> VKVDLESKRYGEKLKEVFLMLDNNVVECIKEITESSRNGKLVFFVGAGVSTLSDYPQWWRLVDKYHEELYGSPKKGNYSSDEYLRIPQIFYNVKGEMAFDGILKDFFQVDKPTNPIHDKILAMNPAHVITTNYDNLIDTACW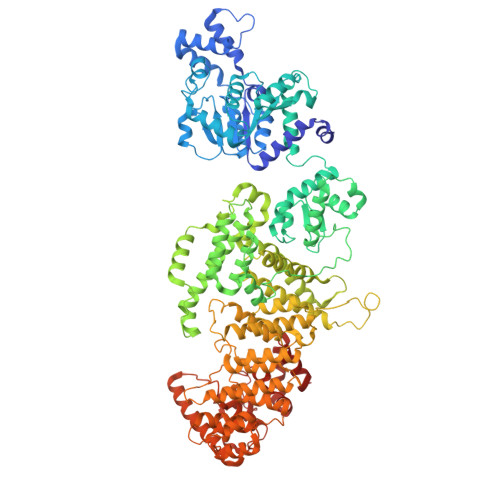KRGKYFSVISAEEDVANATSSRYLLKVHGDFRKGFKGENVVLKEDDYLNYDQNYPLISNLMKTIIATHTIVFIGYGLGDYNINMLLNWVRKLQKDSFHKPFFIRTDPSPIENETLIYYENKGLRIIDAASLIDSNEYDYLERYSAVMDLLIESQENKFITKDDEVIDYIYGKISPLFALQYIRKIDLKHVFEYDYHFEVNGTVVRHKNKGFGYMERFFELKESCDERSKLSKKQYERFNALFNFFEKNGVICMAKDAGTLNTSIEINSLAYHGKYDVMKKFIEEQSVSIEDDYKKAFFLACLGRWEESYDLYSNIILNSIDESNGCVYYLSQINRYRIYQSITQAVTQFNGLGLLTFGRHYKPFTDEFLARIEREMTNFNIDDLFNGMPFEFQKKYKILEFLSDNQFLYDDTVKLFELTNKVRSEMSEGSYSFGMSSDIVVLLRLYDNLRFLYENCLWSVSFHEFHQYIRNSMSLLIEKAEYERTRDIDELGFSFFGKKSGFFMEYYDFVNISRHFKIDDIKNLERSCSIDKIRFGEQEKIEEYLVGIAEEITKQFSANGMNVVFYTQFISEAKAALYFAKYVKLSEEGLGKIVKALLFYFPERDLDIGKRYVWLERLTKCNELPKSIISIIDDFLVLQAEKHIDQNYSEVSSNGLYSRDYGALIKHFEKNFISKRLSEITLCLTQDKQKQIDFLFKLLPLLSTNAKSHLLSFKSVENINDLMNGIRIGLIDEFTPEHEELIIEYLETRKVNYIVEKEKGIQTFSSNDYMSTFGIWYFLEEINNSKMEEFIGMDDQYDFFVDPENFDYKKFIPSWLKNYNDKLLGKIAGNKHMKHHVIEVLKERVKNSNDKRYLEILMNYFI>[4x]MLYLTQRLEIPAAATASVTLPIDVRVKSRVKVTLNDGRDAGLLLPRGLLLRGGDVLSNEEGTEFVQVIAADEEVSVVRC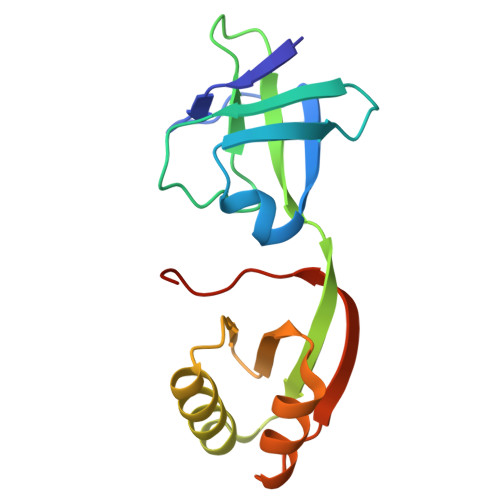DDPFMLAKACYALGNRHVPLQIMPGELRYHHDHVLDDMLRQFGLTVTFGQLPFEPEAGAYASES>[2x]METIQELILSEENKTNIAVLNLGTNDRRNAVLILETALHLVEKYLGKIINTSYLYETVPEYIVLDKKESCEKINKDCRIYDVNYINELMQNLEESKYEENKELIDKCEEYETFLKNGKVDNSILKEVNVENYLLECNNIIVKNDEIMKNNLSKYKDKYYTSYFYNLTVVVKTFVNDPLSMLVVIKYIEELMKRENVKEKEKFENRIIDIDILFFNDFTIFMKNIKLEKNMIYKILSKYIHLERDIKNGNDNMSKVNMDKDINLNNNNNIKKKNNNDIDCDCVDQKMNNHVN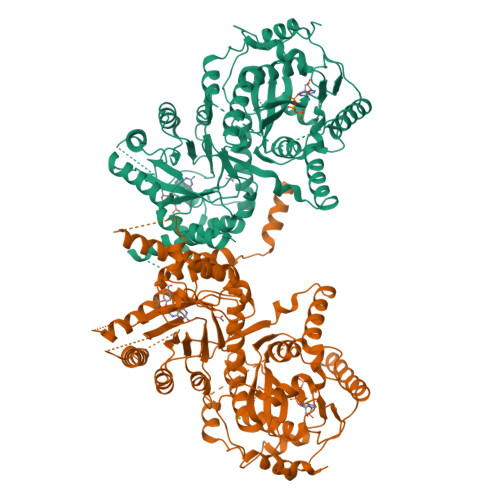NKNYINSFRDPQEIINNMVDNIEFLSIPHVYTTHRYSILLCLNDMIPEYKHNVLNNTIRCLYNKYVSRMKEQYNINIKENNKRIYVLKDRISYLKEKTNIVGILNVNYDSFSDGGIFVEPKRAVQRMFEMINEGASVIDIGGESSGPFVIPNPKISERDLVVPVLQLFQKEWNDIKNKIVKCDAKPIISIDTINYNVFKECVDNDLVDILNDISACTNNPEIIKLLKKKNKFYSVVLMHKRGNPHTMDELTNYDNLVYDIKNYLEQRLNFLVLNGIPRYRILFDIGLGFAKKHDQSIKLLQNIHVYDEYPLFIGYSRKRFIAHCMNDQNVVINTQQKLHDEQQNENKNIVDKSHNWMFQMNYMRKDKDQLLYQKNICGGLAIASYSYYKKVDLIRVHDVLETKSVLDVLTKIDQVKDPNSSSVDKLAAALEHHHHHH> AALPDQSFLWNVFQRVDKDRSGVISDTELQQALSNGTWTPFNPVTVRSII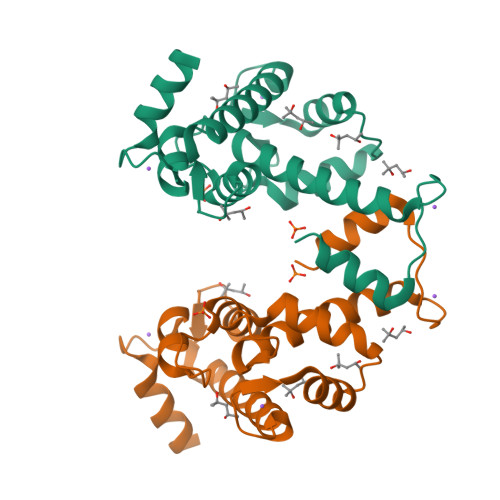SMFDRENKAGVNFSEFTGVWKYITDWQNVFRTYDRDNSGMIDKNELKQALSGFGYRLSDQFHDILIRKFDRQGRGQIAFDDFIQGCIVLQRLTDIFRRYDTDQDGWIQVSYEQYLSMVFSIV> MPTYEELSQAVFEGDEAQVVELTRSLLSGGAEPLEVINKGLIAGMDRVGVLFKNNEMFVPEVLMSANAMNAGVEVVKQSQQAFDMPSVGKIVLGTVKGDLHDIGKNLVAMMLESGGFTVYNLGVDIEPGKFVEAVKKYQPDIVGMSALLTTTMMN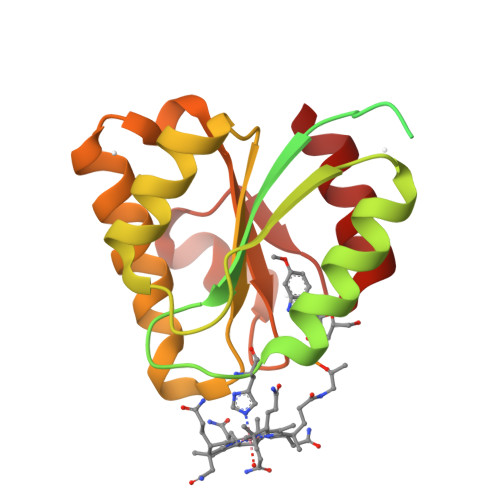MKSTIDALIAAGLRDRVKVIVGGAPLSQDFADEIGADGYAPDAASATELCRQLLE>SAKDERAREILRGFKLNWMNLRDAETGKILWQGTEDLSVPGVEHEARVPKKILKCKAVSRELNFSSTEQMEKFRLEQKVYFKGQCLEEWFFEFGFVIPNSTNTWQSLIEAAPESQMMPASVLTGNVIIETKFFDDDLLVSTSRVRLFYV[2x];> SGPGCMSCKC

RAS is a major anticancer drug target which requires membrane localization to activate downstream signal transduction. Phosphodiesterase 6δ (PDE6D) has a beta-sandwich immunoglobulin fold which contains a hydrophobic pocket capable of binding to the farnesyl group. PDE6D binds to and sequesters the lipid of cytoplasmic RAS and has been proposed to deliver GTPase to recycling endosomes, which is followed by release mediated by the small G-protein Arf-like 2 (ARL2), allowing RAS to be trafficked back to the plasma membrane. The resultant lipid modification increases the affinity of RAS proteins toward membranes, where it is required for signal transduction. Here, we present a novel strategy for targeting RAS by stabilizing its interaction with the prenyl-binding protein PDE6D and disrupting its localization.

Within their HVR sequences, both HRAS and NRAS contain a cysteine residue in the −5 position relative to the modified C-terminal cysteine. HRAS has an additional cysteine residue in the −2 position. We were successfully able to cocrystallize PDE6D with C-terminally modified peptides of both HRAS and NRAS. The crystal structure containing HRAS peptide contains two copies of the complex, each in a different conformation. In one complex, the density is readily interpreted for six amino acids including both cysteine residues, while in the second PDE6D:HRAS complex, only the carboxymethylated farnesylated C-terminal cysteine can be confidently modeled. As the electron density for only one copy of the HRAS peptide can be modeled, it suggests that HRAS, like KRAS, has conformational heterogeneity when bound to PDE6D. The cysteine residue in the −5 position is packed against PDE6D and not solvent-exposed —whether this would occur with the full-length HRAS or this result is due to the potential increase in flexibility with a peptide is uncertain. As the −2 cysteine is solvent-exposed, it is possible that it could be targeted with an irreversible small molecule. In summary, HRAS contains two cysteine residues within the HVR, of which at least one (and possibly both) is solvent-exposed and so could be targeted to develop an irreversible inhibitor.>MT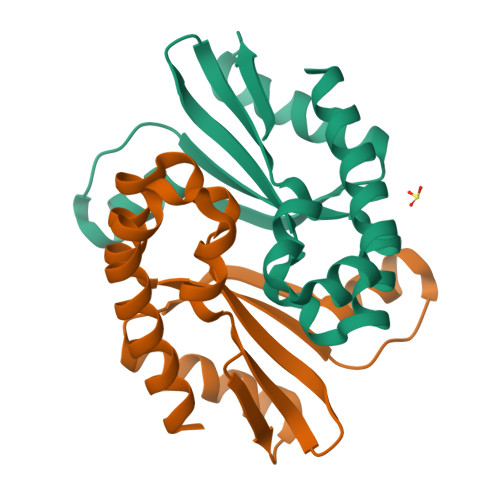GMRKTLKATLAEARAQVEAALKEEGFGILTEIDVAATLKAKLGLEKPPYLILGACNPNLAARALEALPEIGLLLPCNVVLREAEEGVEVLIQDPKEMFRVLPEATQRALAPVAEEARTRLSRALSRL[2x]>DVSGTVCLSALPPEATDTLNLIASDGPFPYSQDGVVFQNRESVLPTQSYGYYHEYTVITPGARTRGTRRI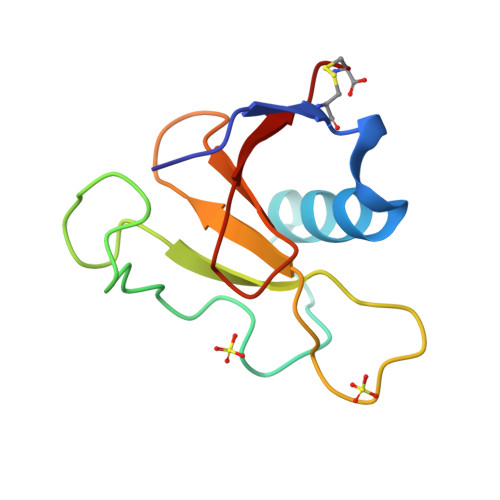ITGEATQEDFYTGDHYATFSLIDQTC[2x]> AIKKDQKAPIITIFDNRGCEVKKNNYSGAKANGMEDDQCVKLTMETITVSETTAAKKLQEFIGLKATAINVPQISGVTKKY;>FSRVVTNADSKAAYVGGADLQALKKFVSEGNKRLDAVNAIVSNASCIVSDAVSGMICENPALISPSGNCYTNRRMAACLRDAEIILRYVSYSLLSGDSSVLEDRCLSGLKETYSSLGVPTAGNLRAVGIMKATCVAFINNTSQQKKLSTPAGDCSALASEVAGYFDKVSAALA[2x];> AIKKDQKAPVVT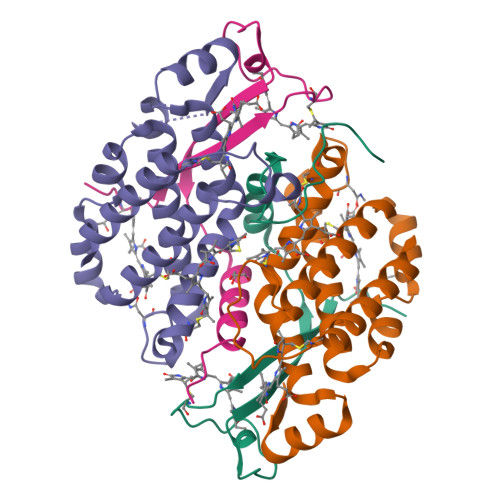IFDARGCKDHSNKEYTGAKAGGMEDDQCVKLTMETIKVGDDVAAKVLGECLSELKSRK> MRKFILSLSILLSALLVACSSRNHYGDTGSLAGLQAMADSKYTRAQKKQKMGKIREMALKETALSVGAQAGLAWRAKIIDEQLNKQARNLDAIYDFNSLVLEHNILPPVLLEGRNTLNLADAQSIRISDRTYKVAKQAHFITTPPTWRQYLWMDYVKPEAPNVTLLPKTKAEKEIWCIYTERGWKNGIDQANTILEENIARIKEDFGGMILYRKLLAMNMVSPPYVS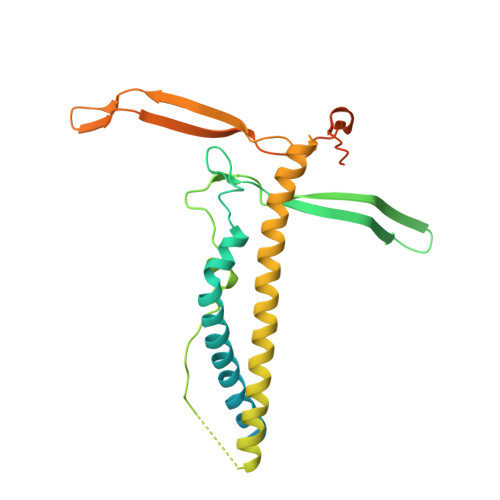HTDLGVTGDGSEIHIDDRVLRITALPELNVNSAEWRAAVAKDENALERFKNMEKLANQAKIVITNKSWQPIIAPVS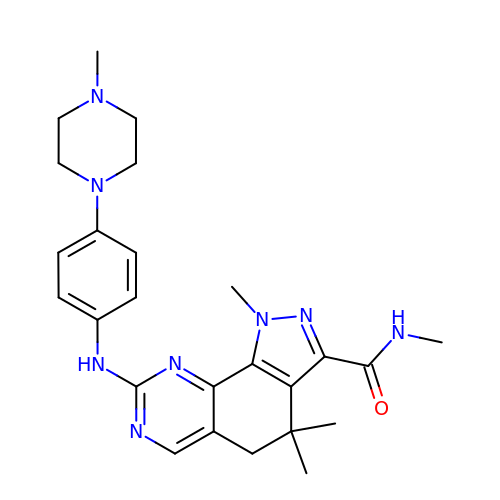N,1,4,4-TETRAMETHYL-8-{[4-(4-METHYLPIPERAZIN-1-YL)PHENYL]AMINO}-4,5-DIHYDRO-1H-PYRAZOLO[4,3-H]QUINAZOLINE-3-CARBOXAMIDE | C25 H32 N8 O | RXZMYLDMFYNEIM-UHFFFAOYSA-N5-CHLORO-N-((1R,2S)-2-(4-(2-OXOPYRIDIN-1(2H)-YL)BENZAMIDO) CYCLOPENTYL)THIOPHENE-2-CARBOXAMIDE | 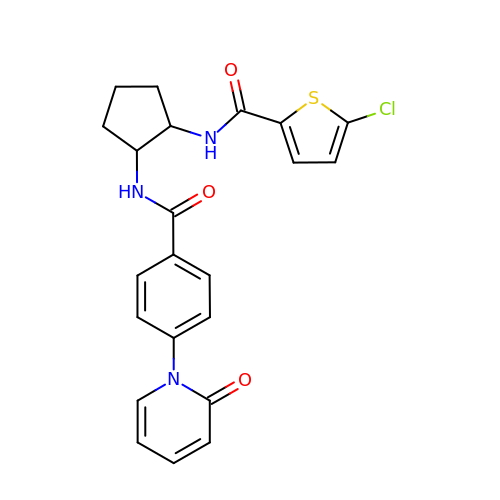C22 H20 Cl N3 O3 S | QCPYHSAHOYXXQK-DLBZAZTESA-N>[30x]GSHMSLIDPRAIIDPSARLAADVQVGPWSIVGAEVEIGEGTVIGPHVVLKGP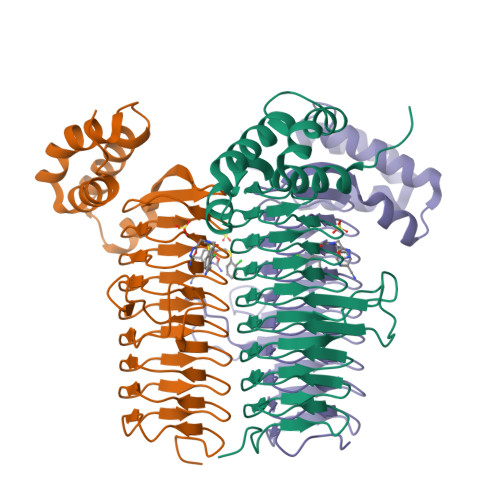TKIGKHNRIYQFSSVGEDTPDLKYKGEPTRLVIGDHNVIREGVTIHRGTVQDRAETTIGDHNLIMAYAHIGHDSVIGNHCILVNNTALAGHVHVDDWAILSGYTLVHQYCRIGAHSFSGMGSAIGKDVPAYVTVFGNPAEARSMNFEGMRRRGFSSEAIHALRRAYKVVYRQGHTVEEALAELAESAAQFPEVAVFRDSIQSATRGITR GIPC1 (GAIP interacting protein, C-terminus 1) and its two paralogs GIPC2 and GIPC3 are universal adaptor proteins that bind and regulate vesicular trafficking of many transmembrane proteins. GIPCs contribute to the endocytosis process by tethering the cargo proteins on endocytic vesicles to the motor protein myosin VI. GIPCs contain a central PDZ (PSD-95, Dlg and ZO-1) domain that mediates the interaction with the C-terminal PDZ-binding motif (PBM) in cargo proteins. The transmembrane receptor PlexinD1 contains a C-terminal ‘SEA’ motif that constitutes a PBM and interacts with GIPC1.

We determined the crystal structures of the myosin VI-HCBD in complex with the GH2 domain from GIPC1 and GIPC2, respectively. There are five copies of both myosin VI-HCBD and GIPC1-GH2 molecules in each asymmetric unit, arranged in an alternating pattern. The group of five HCBD and GH2 domains repeats itself in the neighboring unit cell, yielding a continuous array of alternating HCBD and GH2 that extends throughout the crystal. Considering one GH2/HCBD pair as a unit, the neighboring units in the array are related roughly by a five-fold right-handed rotational symmetry and a ~22 Å translation. The bivalent interactions between the GIPC-GH2 and myosin VI-HCBD are mediated by two distinct interfaces. Interface I involves the two loops in the GIPC-GH2 domain, one between helices α1 and α2 and the other between helices α3 and α4. These two loops interact with Arg1084 and Arg1085 in the ‘RRL’ motif on one side of the second helix in the myosin VI-HCBD. In addition, hydrophobic residues such as Val1088, Tyr1089 and Trp1092 on the same side of the second helix in the myosin VI-HCBD dock on the hydrophobic patch formed by Tyr275, Met276, Ile278, Leu283, Phe311, etc. in the GIPC1-GH2 domain. Interface II is formed on the opposite side of the HCBD with helix α4 and the N-terminal end of helix α3 in the GIPC1-GH2 domain. Interfaces I and II bury ~1300 and ~1100 Å2 solvent accessible surface area, respectively.

>[5x]GPHMSAFEEKAIEKVDDLLESYMGIRDTELAATMVELGKDKRNPDELAEALDERLGDFAFPDEFVFDVWGAIGDAKVGRY;>GPGSHDLSKWKYAELRDTINTSCDIELLAACREEFHRRLKVYHAWKSKN[5x]>[4x]MRLLVGNDWSEELAEPTGSTGWAVQRLVWFARDGDVLVLPVAPQEEFLAYVTSLTGTRRSSLTVVVPPPGRLGAGALTADRL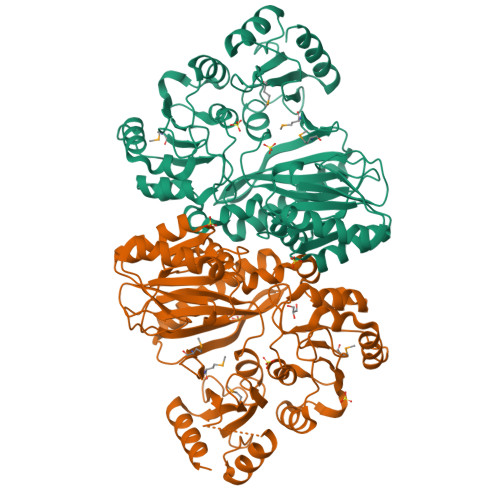ADPRFLAALREAFAGRPVHEVFALWPDAVVADLADALGCPEALEGHDFLTQSGGLIGSSKAAFRALAAGAGVALPAGAVCADRRRAHRHVTRLLDEGSPVILKQDYGSGSDGNEILSRTPGLALRGARALRVLADSAALDAYLDERWDWLTEGGRHRVVVERYHPGSRAYFAEFWISDGGVRLGGHGEMRYRPLPDSQVMPAPDLDQAQLDDLVEGGRRLCVALHALGYRGVLSADAVVTPAGEVLFTEHNGRATGSTHIYEIVGKRVVGPGFGTDRILLERVWPEGWEAPSFAGALTRLRDSGHLYDPETRRGAVILAAYNTHRKGVMLCYVAEDLEAALHREESVSRLFAPALSALEHHHHHH>[12x]MRGSHHHHHHGSLVPRGSMVSVIKPDMKIKLRMEGAVNGHPFAIEGVGLGKPFEGKQSMDLKVKEGGPLPFAYDILTTVFSYGNRVFAKYPENIVDYFKQSFPE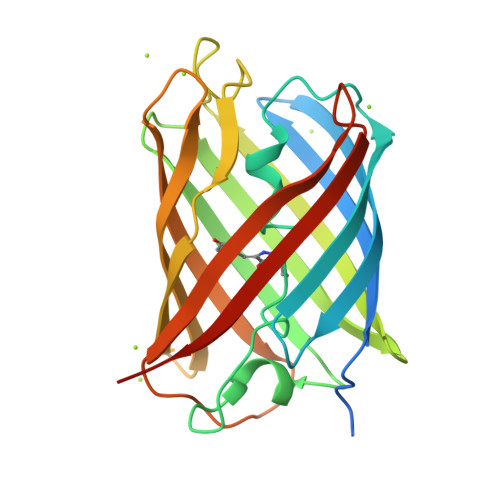GYSWERSMNYEDGGICNATNDITLDGDCYIYEIRFDGVNFPANGPVMQKRTVKWEPSTEKLYVRDGVLKGDVNMALSLEGGGHYRCDFKTTYKAKKVVQLPDYHFVDHHIEIKSHDKDYSNVNLHEHAEAHSELPRQAK> ALEEAPWPPPEGAFVGFVLSRKEPMWADLLALAAARGGRVHRAPEPYKALRDLKEARGLLAKDLSVLALREGLGLPPGDDPMLLAYLLDPSNTTPEGVARRYGGEWTEEAGERAALSERLFANLWGRLEGEERLLWLYREVERPLSAVLAHMEATGVRLDVAYLRALSLEVAEEIARLEAEVFRLAGHPFNLNSRDQLERVLFDELGLPAIGKTEKTGKRSTSAAVLEALREAHPIVEKILQYRELTKLKSTYIDPLPDLIHPRTGRLHTRFNQTATATGRLSSSDPNLQNIPVRTPLGQRIRRAFIAEEGWLLVALDYSQKELRVLAH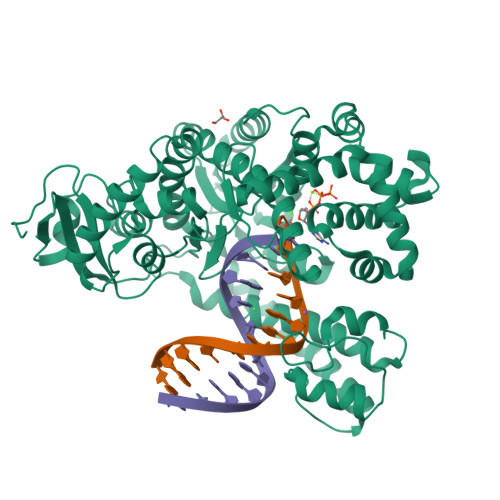LSGDENLIRVFQEGRDIHTETASWMFGVPREAVDPLMRRAAKTINFGVLYGMSAHRLSQELAIPYEEAQAFIERYFQSFPKVRAWIEKTLEEGRRRGYVETLFGRRRYVPDLEARVKSVREAAERKAFNMPVQGTAADLMKLAMVKLFPRLEEMGARMLLQVHDELVLEAPKERAEAVARLAKEVMEGVYPLAVPLEVEVGIGEDWLSAKE> QCNGIYIWKIGNFGMHLKCQEEEKPVVIHSPGFYTGKPGYKLCMRLHLQLPTAQRCANYISLFVHTMQGEYDSHLPWPFQGTIRLTILDQSEAPVRQNHEEIMDAKPELLAFQRPTIPRNPKGFGYVTFMHLEALRQRTFIKDDTLLVRCEVSTRFDL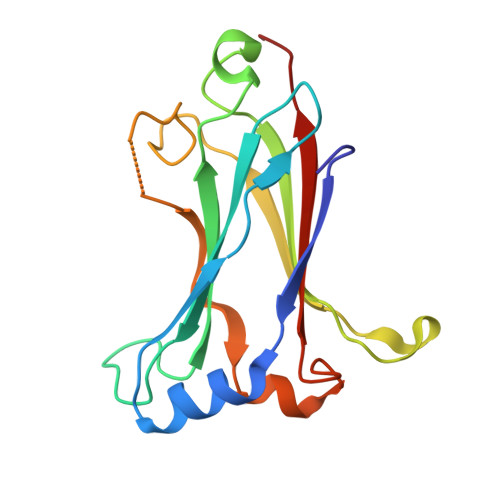E>GPLGSSSGQSNNNSDTCAEFRIKYVGAIEKLKLSEGKGLEGPLDLINYIDVAQQDGKLPFVPPEEEFIMGVSKYGIKVSTSDQYDVLHRHALYLIIRMVCYDDGLGAGKSLLALKTTDASNEEYSLWVYQCNSLEQAQAICKVLSTAFDSVLTSEKP[32x]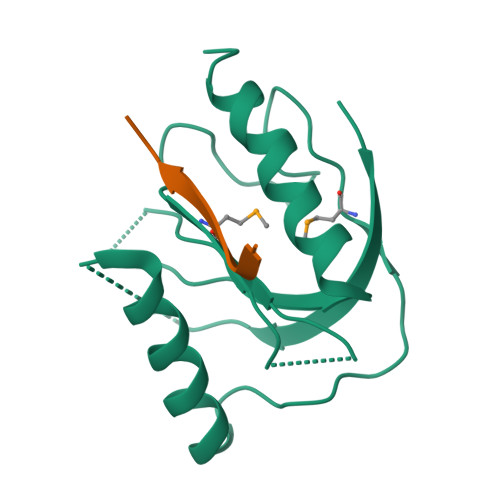;>KSAVTTVVNPKYEGK[30x]>[3x]MPEGPELHLASQFVNEACRALVFGGCVEKSSVSRNPEVPFESSAYRISASARGKELRLILSPLPGAQPQQEPLALVFRFGMSGSFQLVPREELPRHAHLRFYTAPPGPRLALCFVDIRRFGRWDLGGKWQPGRGPCVLQEYQQFRENVLRNLADKAFDRPICEALLDQRFFNGIGNYLRAEILYRLKIPPFEKARSVLEALQQHRPSPELTLSQKIRTKLQNPDLLELCHSVPKEVVQLGGRGHGSESGEEDFAAFRAWLRCYGMPGMSSLQDRHGRTIWFQGDPGPLAPKGRKS

Human endonuclease VIII-like 1 (hNEIL1) is a bifunctional DNA glycosylase of the Fpg/Nei family, which catalyzes the removal of damaged bases and subsequent incision of the newly generated abasic sites. Unlike traditional enzymes which are commonly referred to as highly specific biocatalysts, one special feature for hNEIL1 is its unique capability to recognize a wide range of substrates, including formamidopyrimidines, hydantoin lesions, oxidized, and dihydro-modified pyrimidine bases, derived from all four canonical bases. Here, by integrating structural, computational, and biochemical investigations, we show that hNEIL1 uses a triage mechanism to achieve broad specificity and reduce futile repair of normal bases. This mechanism involves two mutually competing interaction states: an activated state that commits catalysis and BER, and a quarantine state that temporarily separates and prevents the flipped base from catalysis via auto-inhibition.

We synthesized a 2′-fluoro-substituted stable mimic of DHU (FDHU), which allows binding but not catalysis by hNEIL1. In light of the observation that different hNEIL1–DNA interaction modes are largely resulted from the conformation changes of the lesion recognition loop, we chose to modify the potential key amino acids on this loop. In order to destabilize the quarantine state, we rationally designed hNEIL1(R242, G249P) and hNEIL1(R242, Y244H) to disrupt the flexibility of the loop or the aromatic stacking interactions respectively. Instead of the quarantine state originally observed in hNEIL1(R242)–FDHU structure, we found that both two mutants switched to the activated state as expected. Our study reveals that instead of utilizing a specific pocket to tightly recognize a flipped base via extensive electrostatic and hydrogen bonding interactions, hNEIL1 uses two competing interaction states to achieve substrate recognition. This mechanism is further corroborated by our finding that the relative dominance of the competing interaction states can be manipulated by artificially introduced or naturally existing mutations to the key lesion recognition loop.> GIDPFTIRSNRTEGQALLSDAAARQERYYSQNPGVGYTKDVAKLGMSSANS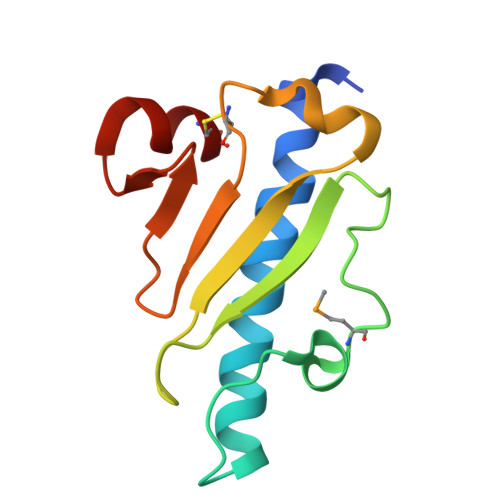PNNLYNLTIATPTSTTYTLTATPINSQTRDKTCGKLTLNQLGERGAAGKTGNNSTVNDCWR> MPTVDDILEQVGESGWFQKQAFLILCLLSAAFAPICVGIVFLGFTPDHHCQSPGVAELSQRCGWSPAEELNYTVPGLGPAGEAFLGQCRRYEVDWNQSALSCVDPLASLATNRSHLPLGPCQDGWVYDTPGSSIVTEFNLVCADSWKLDLFQSCLNAGFLFGSLGVGYFADRFGRKLCLLGTVLVNAVSGVLMAFSPNYMSMLLFRLLQGLVSKGNWMAGYTLITEFVGSGSRRTVAIMYQMAFTVGLVALTGLAYALPHWRWLQLAVSLPTFLFLLYYWCVPESPRWLLSQKRNTEAIKIMDHIAQKNGKLPPADLKMLSLEEDVTEKLSPSFADLFRTPRLRKRTFILMYLWFTDSVLYQGLILHMGATSGNLYLDFLYSALVE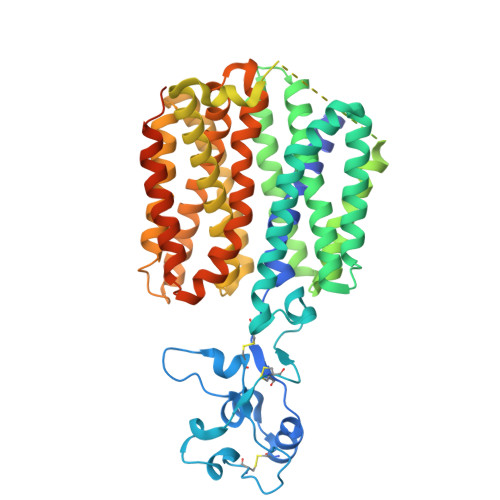IPGAFIALITIDRVGRIYPMAMSNLLAGAACLVMIFISPDLHWLNIIIMCVGRMGITIAIQMICLVNAELYPTFVRNLGVMVCSSLCDIGGIITPFIVFRLREVWQALPLILFAVLGLLAAGVTLLLPETKGVALPETMKDAENLGRKAKPKENTIYLKVQTSEPSGT> RI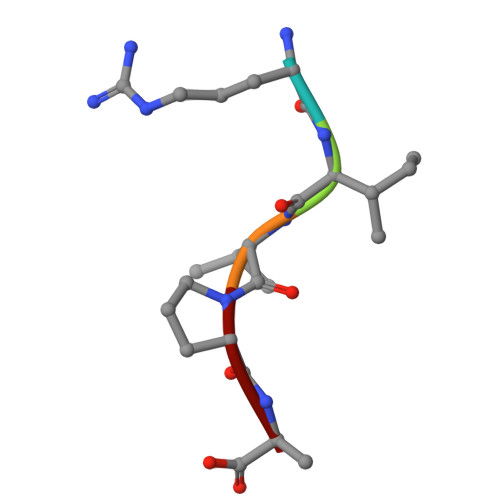VPA> GPKQKIVIKATMSNAKSRAQAMVLASKANGVGSVGITGDLKDQLEVVGVGIDIACLVRCLRKKLRYAEIVKVEEVKDK;> MQNEYLDAKKHGIDLSRERAPNFVDHPGIPPSDCFWFLYKNYVRQDAGVCQSDWSFDMKIGQYWVTIHTDEGCRLSGIIPAGWLILGIKRLGF

Here, we unravelled the biochemical and structural basis of adaptive evolution of APikL2, an exceptionally conserved paralog of the well-studied rice-lineage specific effector AVR-Pik. Whereas AVR-Pik and other members of the six-gene AVR-Pik family show specific patterns of presence/absence polymorphisms between grass-specific lineages of M. oryzae, APikL2 stands out by being ubiquitously present in all blast fungus lineages from 13 different host species. Using biochemical, biophysical and structural biology methods, we show that a single aspartate to asparagine polymorphism expands the binding spectrum of APikL2 to host proteins of the heavy-metal associated (HMA) domain family. The structures were solved and refined as described in the Materials and Methods. In each case, the APikL2 variants and HMAs form 1:1 complexes, with both displaying the same global fold and interaction interfaces as previously described for the interaction of AVR-Pik with the Pik-1 integrated HMA domains.

We crystallized complexes of APikL2F with sHMA94 and APikL2A with sHMA25 following co-expression in E. coli for comparative structural analysis. X-ray diffraction data were collected at the Diamond Light Source (Oxford, UK) to 2.3 Å and 1.8 Å resolution, for APikL2F/sHMA94 and APikL2A/sHMA25, respectively. The APikL2A/sHMA25 structure was solved by molecular replacement using PHASER and the PikpHMA/AVR-PikD structure. The APikL2F/sHMA94 and APikL2A/sHMA25 complexes display the three binding interfaces previously reported for AVR-Pik/HMA complexes. They share similar interface areas of ~964 Å and ~1011 Å (calculated by QtPISA) contributed by 57 and 56 residues, respectively. The APikL2F/sHMA94 and APikL2A/sHMA25 complexes are very similar to each other (they superimpose with root-mean-square-deviation (RMSD) of 0.582 Å across the aligned Cα backbones). The largest differences between the complexes are within interface 3, where APikL2 forms several interactions with sHMA25 that cannot be formed with sHMA94 due to differences in the sequences of the HMAs in this region. The interface 2 region of sHMA94 and sHMA25, which forms contacts with the Asp-66/Asn-66 residues of APikL2, is highly conserved in both complexes. However, we observed that the presence of Asn-66 in APikL2F results in an altered local hydrogen bonding network around Gln-44 in sHMA94, when compared to Asp-66 in the APikL2A/sHMA25 complex. In this orientation, the NE2 atom of Gln-44 interacts with the OG1 atom and backbone carbonyl of Thr-38. This hydrogen bonding arrangement is not adopted in the APikL2A/sHMA25 complex, as the Asp-66 in APikL2A forms a hydrogen bond with the NE2 atom of Gln-43 in sHMA25, rotating the NE2 group away from Thr-37, and preventing formation of hydrogen bonds between these two residues.4-[3-(4-fluorophenyl)-1H-pyrazol-4-yl]-N-[2-(piperazin-1-yl)ethyl]-2-(trifluoromethyl)aniline | C22 H23 F4 N5 | 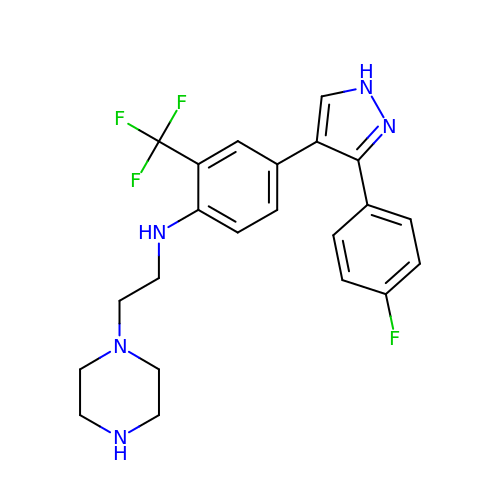OXSJLZKYOPQBJE-UHFFFAOYSA-N(3Z)-3-(1H-IMIDAZOL-5-YLMETHYLENE)-5-METHOXY-1H-INDOL-2(3H)-ONE | C13 H11 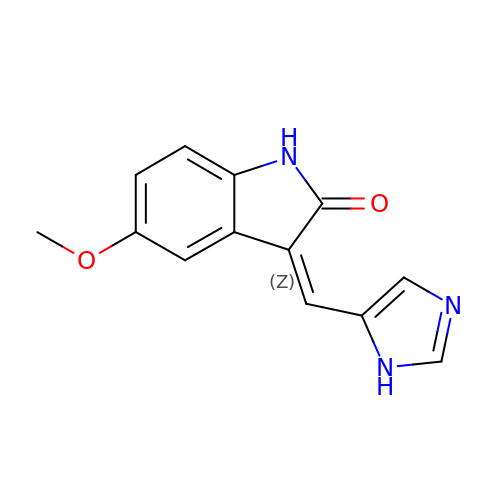N3 O2 | QNUKRWAIZMBVCU-WCIBSUBMSA-N> MHHHHHHENLYFQSMASGTTTTAVKIGIIGGTGLDDPEILEGRTEKYVDTPFGKPSDALILGKIKNVDCVLLARHGRQHTIMPSKVNYQANIWALKEEGCTHVIVTTACGSLREEIQPGDIVIIDQFIDRTTMRPQSFYDGSHSCARGVCHIPMAEPFCPKTREVLIETAKKLGLRCHSKGTMVTIEGPRFSSRAESFMFRTWGADVINMTTVPEVVLAKEAGICYASIAMATDYDCWKEHEEAVSVDRVLKT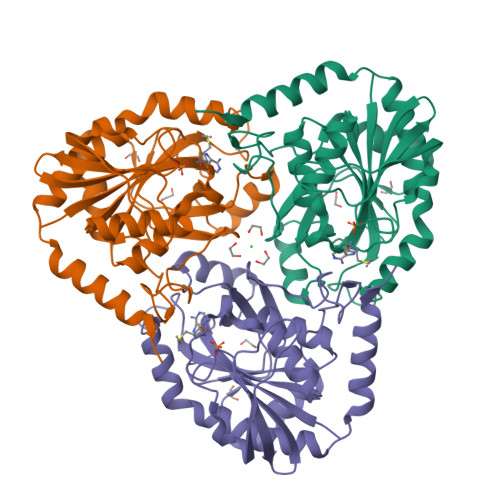LKENANKAKSLLLTTIPQIGSTEWSETLHNLKNMAQFSVLLPRH> MSDLQDQEPSIIINGNLEPVGEPDIVEETEVVAQETQETQDADKPKKKVAFTGLEEDGETEEEKRKREFEEGGGLPEQPLNPDFSKLNPLSAEIINRQATINIGTIGHVAHGKSTVVRAISGVQTVRFKDELERNITIKLGYANAKIYKCQEPTCPEPDCYRSFKSDKEISPKCQRPGCPGRYKLVRHVSFVDCPGHDILMSTMLSGAAVMDAALLLIAGNESCPQPQTSEHLAAIEIMKLKHVIILQNKVDLMREESALEHQKSILKFIRGTIADGAPIVPISAQLKYNIDAVNEFIVKTIPVPPRDFMISPRLIVIRSFDVNKPGAEIEDLKGGVAGGSILNGVFKLGDEIEIRPGIVTKDDKGKIQCKPIFSNIVSLFAEQNDLKFAVPGGLIGVGTKVDPTL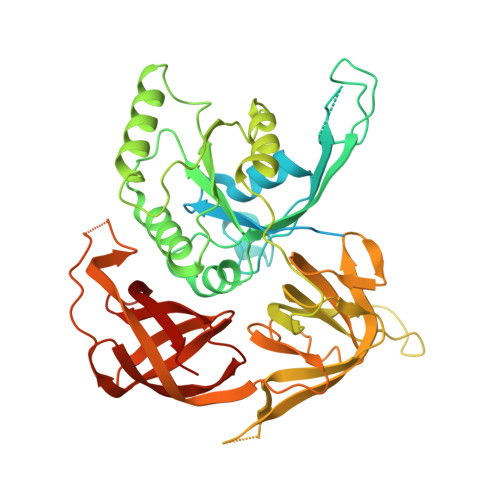CRADRLVGQVVGAKGHLPNIYTDIEINYFLLRRLLGVKTDGQKQAKVRKLEPNEVLMVNIGSTATGARVVAVKADMARLQLTSPACTEINEKIALSRRIEKHWRLIGWATIKKGTTLEPIA>MNRDIGKNAERELVSILRGEGFNAVRIPTSNSSPNPLPDIFATKGNTLLSIECKSTWENKVKVKEHQVRKLLDFLSMFTMKGVPLIAIKFKQVHEWRVLVPEKAEDIIVTIDNSIPIEDLFKILEKRIEEKILT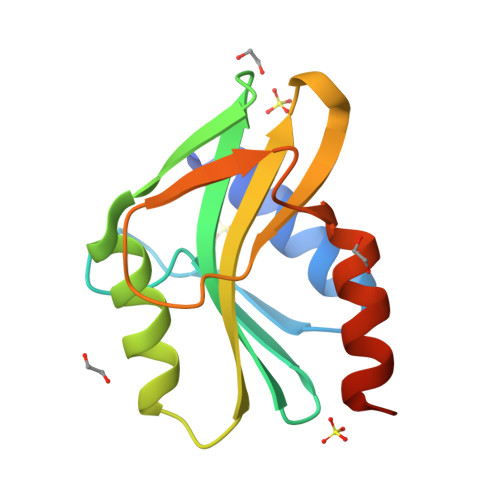P[2x]> TEQTLFEQLNSKNVNDHTEQKNGLTYLAWSYAHQELKKIDPNYTVKVHEFPHPDINTENYFVPYLATPEGYFVQVSVTVKDSTETEWLPVLDFRNKSLAKGSATTFDINKAQKRCFVKASALHGLGLY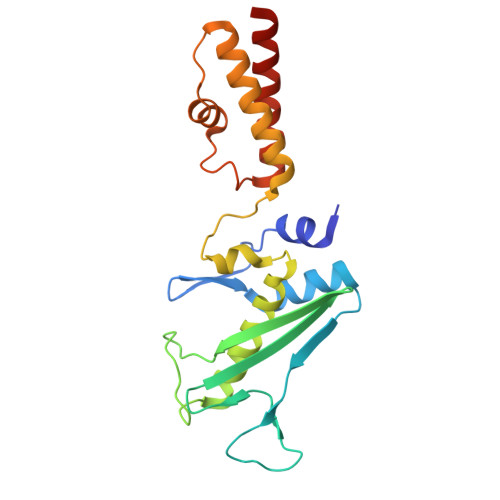IYNGEELPSASDNDITELEERINQFVNLSQEKGRDATIDKTMRWLKISNINKLSQKQIAEAHQKLDAGLKQLDSEEKQ> GPLGSQFLVYKNIIKDYIQSRLFNEGLLDGPYRCDIKDVKTKKVSERLKEVG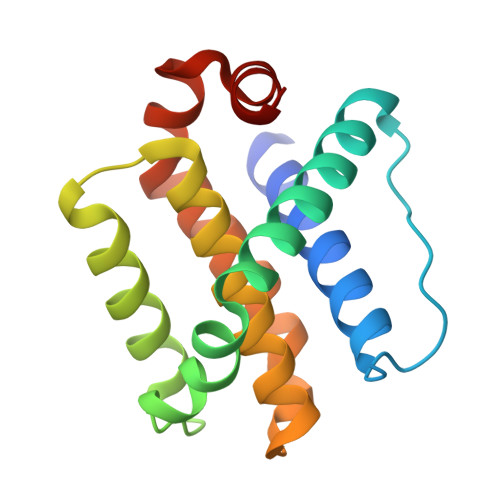NELEGKFKDSFSNMCERLTITDTTAYPTFVGVVNELFSTGINWGRIVAFIVFSSRLAIHFKRNGMPEYVKSVYGWVARYMHTKLSTWIEANRSWDGFLDHFD> EAEAHHHHHHLANTSAHDFSYLKFVYNATDTSLEGSYDYIVIGGGTSGCPLAATLSEKYKVLLLERGTIATEYPNTLTADGFAYNLQQQDDGKTPVERFVSEDGIDNVRARILGGTTIINAGVYARANISFYSQTGIEWDLDLVNKTYEWVEDAIVVKPNNQSWQSVIGEGFLEAGILPDNGFSLDHEAGTRLTGSTFDNNGTRHAADELLNKGDPNNLLVAVQASVEKILFSSNTSNLSAIGVIYTDSDGNSHQAFVRGNGEVIVSA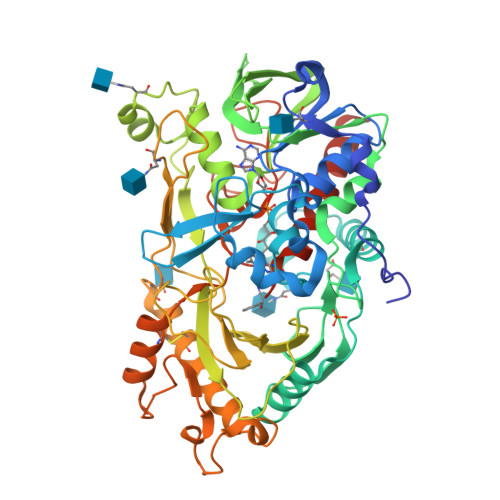GTIGTPQLLLLSGVGPESYLSSLNITVVQPNPYVGQFVYDNPRNFINILPPNPIEASVVTVLGIRSDYYQVSLSSLPFSTPPFSLFPTTSYPLPNSTFAHIVSQVPGPLSHGSVTLNSSSDVRIAPNIKFNYYSNSTDLANCVSGMKKLGDLLRTKALEPYKARDVLGIDGFNYLGVPLPENQTDDASFETFCLDNVASYWHYHGGSLVGKVLDDSFRVMGIKALRVVDASTFPYEPNSHPQGFYLMLGRYVGLQILQERSIRLEAIHNIQESM> MLRLSAPGQLDDDLCLLGDVQVPVFLLRLGEASWALVEGGISRDAELVWADLCRWVADPSQVHYWLITHKHYDHCGLLPYLCPRLPNVQVLASERTCQAWKSESAVRVVERLNRQLLRAEQRLPEACAWDALPVRAVADGEWLELGPRHRLQVIEAHGHSDDHVVFYDVRRRRLFCGDALGEFDEAEGVWRPLVFDDMEAYLESLERLQRLPTLLQLIPGHGGLLRGRLAADGAESAYTECLRLCRRLLWRQSMGESLDELSEELHRAWGGQSVDFLPGELHLGSMRRMLEI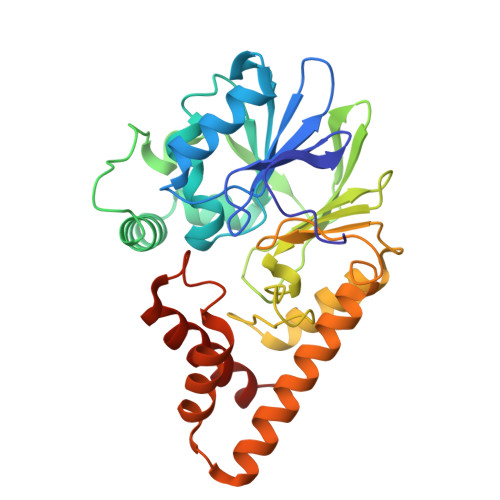LSRQALPLD2-[(2E,6E,10E,14E,18E,22E,26E)-3,7,11,15,19,23,27,31-OCTAMETHYLDOTRIACONTA-2,6,10,14,18,22,26,30-OCTAENYL]PHENOL 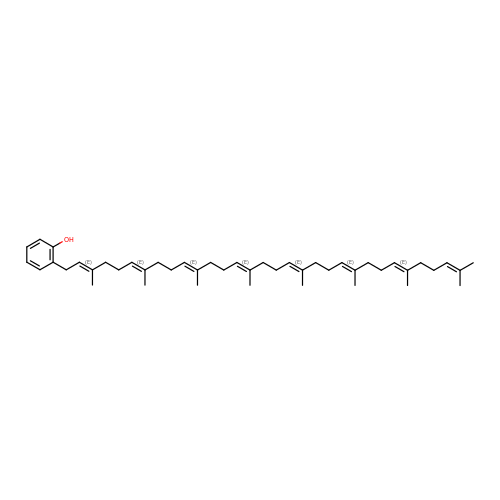| C46 H70 O | VUNQJPPPTJIREN-CMAXTTDKSA-N> MAHHHHHHMNLHQTVEHEAAAAFAAAGIAGSPVVLQPTKNAEHGDFQINGVMGAAKKAKQNPRELAQKVADALAGNAVIESAEVAGPGFINLRLRHEFLAQNIHAALNDARFGVAKTAQPQTVVIDYSSPNLAKEMHVGHLRSSIIGDSISRVLEFTGNTVIRQNHVGDWGTQFGMLVAYLVEQQKDNAAFELADLEQFYRAAKVRFDEDPAFADTAREYVVKLQGGDETVLALWKQFVDISLSHAQAVYDTLGLKLRPEDVAGESKYNDDLQPVADDLVQKGLAVEDDGAKVVFLDEFKNKEGEPAAFIVQK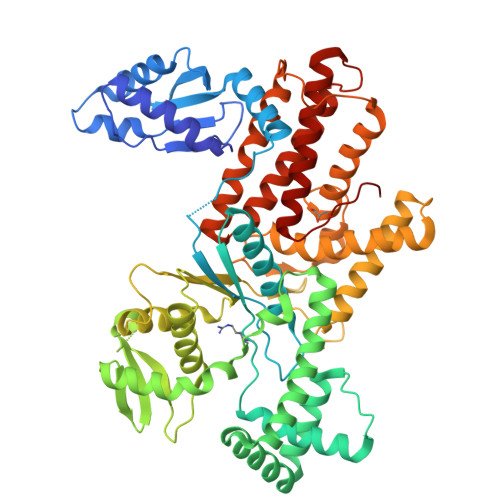QGGGFLYASTDLACLRYRIGRLKAGRLLYVVDHRQALHFEQLFTTSRKAGYLPEDAKAEFIGFGTMMGKDGKPFKTRSGDTVKLVDLLTEAVERATALVKEKNPELGADEAAKIGKTVGIGAVKYADLSKNRTSDYVFDWDAMLSFEGNTAPYLQYAYTRVQSVFRKAGEWDATAPTVLTEPLEKQLAAELLKFENVLQSVADTAYPHYLAAYLYQAATLFSRFYEACPILKAEGASRNSRLQLAKLTGNTLKQGLDLLGIDVLDVM> SAWRKAGMSYAAYLNVAAQAIRSSL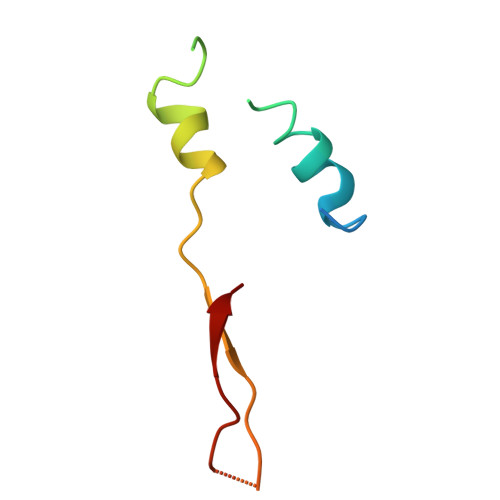KTELQTASVTNRSQTDAFYTQYKNGTAASEPTPMTK> HKPEPTDEEWELIKTVTEAHVATNAQGSHWKQKRKFLPEDIGQAPIVNAPEGGKVDLEAFSHFTKIITPAITRVVDFAKKLPMFCELPCEDQIILLKGCCMEIMSLRAAVRYDPESETLTLNGEMAVTRGQL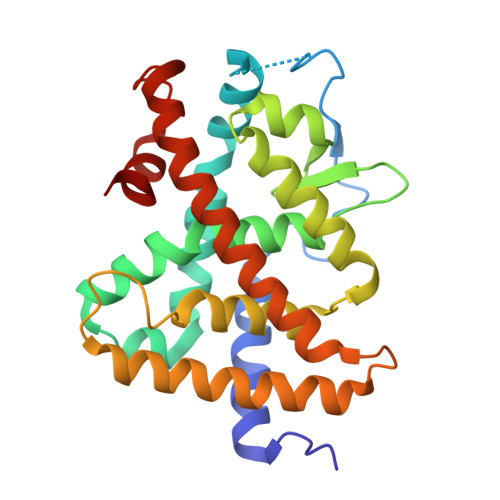KNGGLGVVSDAIFDLGMSLSSFNLDDTEVALLQAVLLMSSDRPGLACVERIEKYQDSFLLAFEHYINYRKHHVTHFWPKLLMKVTDLRMIGACHASRFLHMKVECPTELFPPLFLEVFED N-HYDROXY-N-ISOPROPYLOXAMIC ACID | 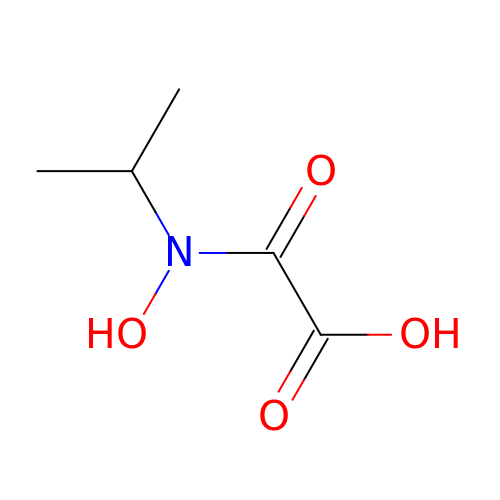C5 H9 N O4 | QVIOSGUKMDGWNN-UHFFFAOYSA-N> SVTVQQPQLTLTAAVIGDGAPANGKTAITVEFTVADFEGKPLAGQEVVITTNNGALPNKITEKTDANGVARIALTNTTDGVTVVTAEVEGQRQSVDTHFVKGTIAADKSTLAAVPTSIIADGLMASTITLELKDTYGDPQAGANVAFDTTLGNMGVITDHNDGTYSAPLTSTTLGVATVTVKVDGAAFSVPSVTVNFTADPIPDAGRSSFTVSTPDILADGTMSSTLSFVPVDKNGHFISGMQ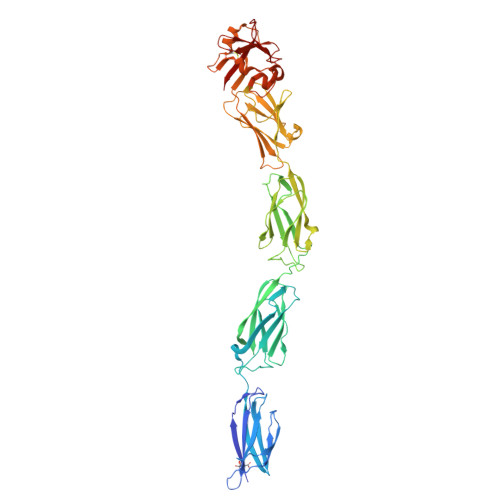GLSFTQNGVPVSISPITEQPDSYTATVVGNSVGDVTITPQVDTLILSTLQKKISLFPVPTLTGILVNGQNFATDKGFPKTIFKNATFQLQMDNDVANNTQYEWSSSFTPNVSVNDQGQVTITYQTYSEVAVTAKSKKFPSYSVSYRFYPNRWIYDGGRSLVSSLEASRQCQGSDMSAVLESSRATNGTRAPDGTLWGEWGSLTAYSSDWQSGEYWVKKTSTDFETMNMDTGALQPGPAYLAFPLCALSI> SFNKQWYLLANQIIQSLSKYEGGHIFEKLVDAKKQNCPDYYDVIKNPMSFSCVKTKLKKGQYGLPTEFIKDVQLIFDNCSLYNTSGSLVAITGKNIEAYFNNQLIVTGYNNFVTKANTINERLQKVEDENLE

In this study, the focus is on the essential Bromodomain protein 1 (PfBDP1) of the malaria pathogen Plasmodium falciparum. Possible targets are the nine predicted bromodomain (BRD) proteins, among which PfBDP1 has been identified as essential in the blood stage of P. falciparum. PfBDP1 is involved in regulating erythrocyte invasion genes and conditional knockdown (KD) of PfBDP1 lead to a significantly reduced multiplication rate during the intraerythrocytic development cycle (IDC). PfBDP1 is recruited to promoters of invasion‐related genes by binding with its BRD to acetylated histones.

Next, we investigated the influence of the meta position. Based on the affinity increase from MPM3 to MPM2, we assumed that hydrophilic groups improve affinity. Based on our models we assumed hydrogen bonds to the side chains of Gln365 and His354 for the sulfonamide variants. Next, we attempted to combine some of the best ortho modifications with some of the best meta or para substituents. Of the combinations tested, three molecules showed improvement over their predecessors. In addition to the interactions described for PfBDP1‐BRD‐RMM2, the structure of RMM21 confirmed the formation of hydrogen bonds to His354 or Gln365 with its sulfonamide, which is present in two conformations. Based on the two conformations of RMM23 in the PfBDP1‐BRD co‐crystal structure, this should be possible for RMM23 and RMM22, but not for RMM21 (compared to RMM20).The ESX-1 type VII secretion system is an important determinant of virulence in pathogenic mycobacteria, including Mycobacterium tuberculosis. This complicated molecular machine secretes folded proteins through the mycobacterial cell envelope to subvert the host immune response. All ESX gene clusters contain at least three or four ESX conserved components (Ecc), named EccB, EccC, and EccD, with EccE being present in all ESX systems with the exception of ESX-4. In this study we report the molecular structures of the periplasmic domain of EccB1 and the cytoplasmic domain of EccD1 from the ESX-1 cluster.

In order to gain further insight into the role of EccB1 within the ESX machinery we determined the crystal structure of the C-terminal domains of EccB1 from M. tuberculosis (EccB1mt) to 1.7 Å resolution and of the orthologous protein (MSMEG_0060; EccB1ms) from the nonpathogenic mycobacterial species M. smegmatis to 3.07 Å resolution. Both EccB1 structures contain a single elongated fold in the shape of a distorted propeller, which has an unanticipated quasi 2-fold symmetry. A structural comparison of the EccB1mt and EccB1ms structures shows that they are highly similar with an r.m.s.d. of 2.7 Å for the superposition of 381 amino acids (Dali Z-score 42.2); there is considerable variability in the conformation of the extensive unstructured loops connecting secondary structure elements which are, themselves, relatively well conserved Five domains are present in the structures including a core domain flanked by two repeat domains on either side. The central core domain consists of a 6 stranded β-sheet with 5 strands (β7-β19-β18-β5-β6) arranged in anti-parallel fashion with an additional strand (β21) parallel to strand β6 on the periphery of the sheet; the sheet is further stabilized by a disulfide bond between the two central strands (β5 and β18) of the sheet formed between Cys150 and Cys345 (EccB1mt) and Cys152 and Cys347 (EccB1ms). Therefore, it appears that R1 is the ancestral domain with R3 sharing more conserved features with R1 than do either R2 or R4. EccB1ms contains a corresponding set of repeats in the same arrangement as seen in EccB1mt: R1 (residues Q75–K127) is membrane proximal, R4 (residues G392–L447), the central core domain, R2 (residues Q187–P243), and R3 (residues G267–E323) which is distal to the membrane. ESX-1 is responsible for secretion of the important virulence factors EsxA and EsxB as well as other virulence-associated proteins (e.g., EspB, EspF, EspJ) that are secreted to the cell surface or extracellular milieu based on recognition of a conserved C-terminal signal sequence on the secretion substrates. These secreted factors have been linked to mycobacterial virulence through studies of the attenuated BCG strain of M. tuberculosis; in non-pathogenic Mycobacterium smegmatis the orthologous ESX-1 system is involved in conjugation.

> SSDQLLVDRTTNQLYVMLPGSNQLRPVYNLTSARLVLGNASNPVAVKSEELNRISKGQSIGIPGAPYATPTGTPASQWTLCDTVAKPDSSAPKVETSILIRTLAIDSGVGPIRADQGMLVSYEGANWLITEGGRHSIDLADRAVTSAVGIPVTAKPTPISQGLFNALPNRGPWQLPQIPAAGAPNSVGLPENLVIGSVFRTATESDPQHYVVLPDGVARVNNTTAAALRATNSYGLMQPPAVEASVVAKIPEQVYVSPLPDQPLDVLLRQDSPVLCWSWQREPGDQAPKTTVIAGRRLPLPANAIGTGIDQIGGDSTVYIEGGQFVRLQSPDPRVGESMYYIDPQGVRYGIANDDAAKNLGLAGPVNAPWQVVGLLVDGPVLSKEAALIEHDTLPADPNPRKVASGEG>LLLMLVLLVAVGQMAQTIYIPAIADMARDLNVREGAVQSVMGAYLLTYGVSQLFYGPISDRVGRRPVILVGMSIFMLATLVAVTTSSLTVLIAASAMQGMGTGVGGVMARTLPRDLYERTQLRHANSLLNMGILVSPLLAPLIGGLLDTMWNWRACYLFLLVLCAGVTFSMARWMPETRPVDAPRTRLLTSYKTLFGNSGFNCYLLMLIGGLAGIAAFEACSGVLMGAVLGLSSMTVSILFILPIPAAFFGAWFAGRPNKRFSTLMWQSVICCLLAGLLMWIPDWFGVMNVWTLLVPAALFFFGAGMLFPLATSGAM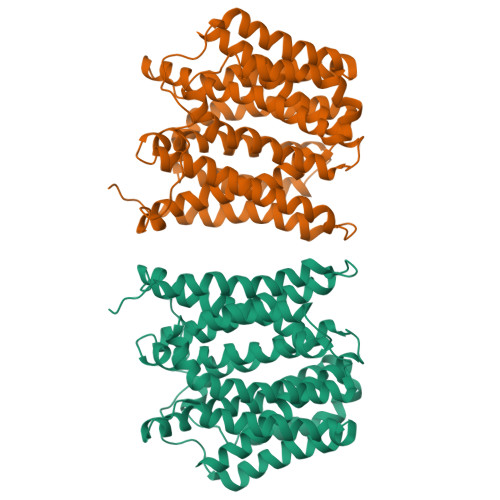EPFPFLAGTAGALVGGLQNIGSGVLASLSAMLPQTGQGSLGLLMTLMGLLIVLCWLPL[2x]> MLRVRCLRGGSRGAEAVHYIGSRLGRTLTGWVQRTFQSTQAATASSRNSCAADDKATEPLPKDCPVSSYNEWDPLEEVIVGRAENACVPPFTIEVKANTYEKYWPFYQKQGGHYFPKDHLKKAVAEIEEMCNILKTEGVTVRRPDPIDWSLKYKTPDFESTGL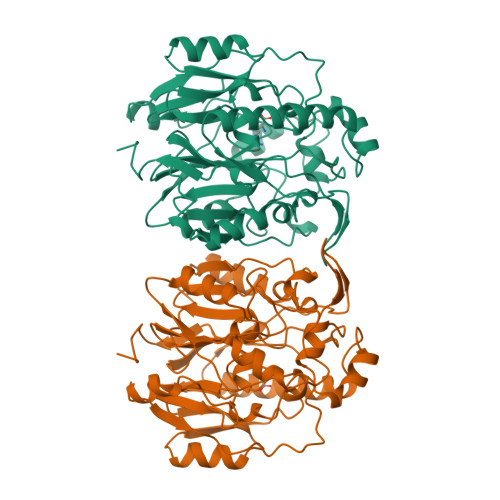YSAMPRDILIVVGNEIIEAPMAWRSRFFEYRAYRSIIKDYFHRGAKWTTAPKPTMADELYNQDYPIHSVEDRHKLAAQGKFVTTEFEPCFDAADFIRAGRDIFAQRSQVTNYLGIEWMRRHLAPDYRVHIISFKDPNPMHIDATFNIIGPGIVLSNPDRPCHQIDLFKKAGWTIITPPTPIIPDDHPLWMSSKWLSMNVLMLDEKRVMVDANEVPIQKMFEKLGITTIKVNIRNANSLGGGFHAWTCDVRRRGTLQSYLD>MDLADRFAELERRYDARLGVYVPATGTTAAIEYRADERFAFCATFKAPLVAAVLHQNPLTHLDKLITYTSDDIRSISPVAQQHVQTGMTIGQLCDAAIRYSDGTAANLLLADLGGPGGGTAAFTGYLRSLGDTVSRLDAEEPELNRDPPGDERDTTTPHAIALVLQQLVLGNALPPDKRALLTDWMARNTTGAKRIRAGFPADWKVIDKTGTGDYGRANDIAVVWSPTGVPYVVAVMSDRAG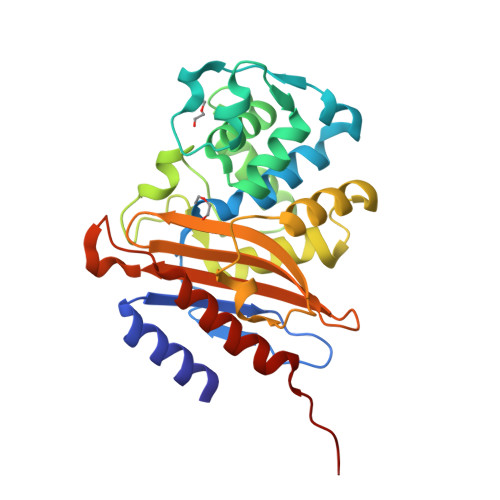GGYDAEPREALLAEAATCVAGVLALEHHHHHH[2x]> MKALIID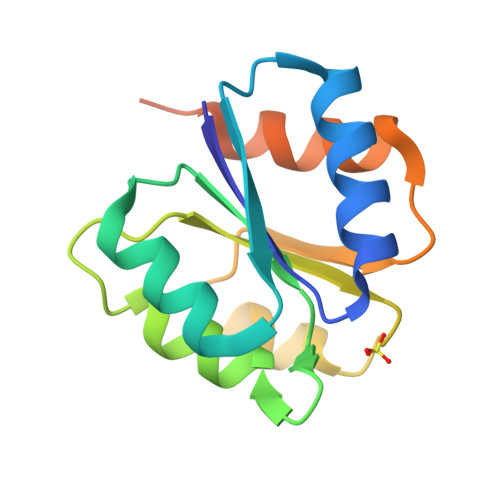DEPLARNELTYLLNEIGGFEEINEAENVKETLEALLINQYDIIFLDVNLMDENGIELGAKIQKMKEPPAIIFATAHDQYAVQAFELNATDYILKPFGQKRIEQAVNKVRATKAKDDNNASAIANDMS> GSHMTIQKVHGREVLDSRGNPTVEVEVTTEKGVFRSAVPSGASTGVYEACELRDGDKKRYVGKGCLQAVKNVNEVIGPALIGRDELKQEELDTLMLRLDGTPNKGKLGANAILGCSMAISKAAAAAKGVPLYRYLASLAGTKELRLPVPCFNVINGGKHAGNALPFQEFMIAPVKATSFSEALRMGSEVYHSLKGIIKKKYGQDAVNVGDE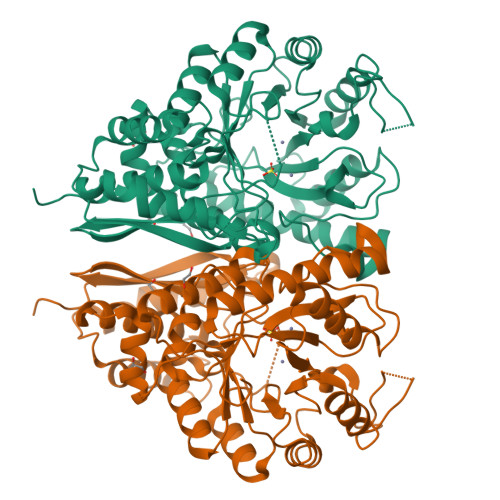GGFAPPIKDINEPLPILMEAIEEAGHRGKFAICMDCAASETYDEKKQQYNLTFKSPEPTWVTAEQLRETYCKWAHDYPIVSIEDPYDQDDFAGFAGITEALKGKTQIVGDDLTVTNTERIKMAIEKKACNSLLLKINQIGTISEAIASSKLCMENGWSVMVSHRSGETEDTYIADLVVALGSGQIKTGAPCRGERTAKLNQLLRIEEELGAHAKFGFPGWS N-[4-[(4R)-1-cyclopentyl-4-methyl-6-oxidanylidene-4,5-dihydropyridazin-3-yl]phenyl]-1,3-dihydropyrrolo[3,4-c]pyridine-2-carboxamide 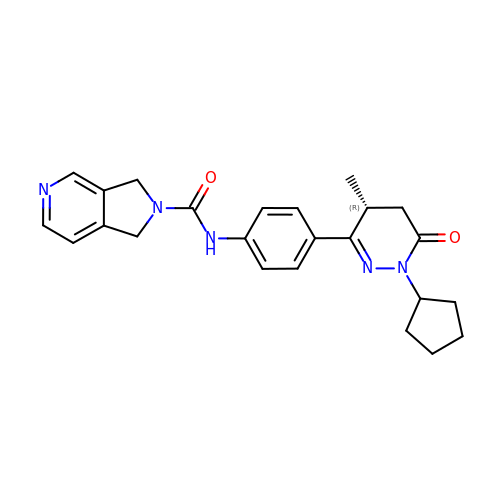| C24 H27 N5 O2 | NMKKGESQLXZFPK-MRXNPFEDSA-N> MILQIHSQNPHLLDLLNKNPHTDLGIYAKSLRNGQLIGNAVSAYQYDVVFQDTRYSYLPEESNQIDFQSYCSPLVILHICNEFFKELLQEKQTYWSQQIKWLERTRAEVDTYPCTIEVKNLYANSTWYSKGHFMMERYFKNIHITPIVGNNLSLRVEGKSVFEAMNLLSFIAVTTHITNTYGEYTYIDDHFAQKYARILTNIPQVPYFVFYLFIKRAIKSERQFAEIKPMFEAYFKEEGLDIDFQFTDTHGSRMDFIVKELGMEYPILDIGCGELKYYRRFMRRNYNYSHPYFATDTDKSVGDYAALLKERMEADNLYFFSDWTDYEYKNPVNIILTEVIEHNTPEAAEALVKHCLSLNFHKMIITTPNSLFNKYYFDEDPESLRHEDHHFEWTPQEFQDFIRHCVGDTSLEV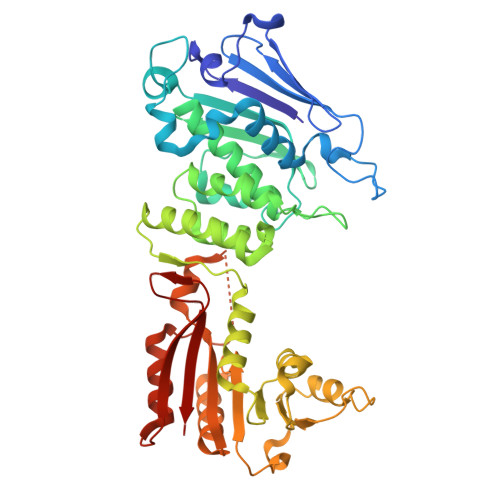TYCGIGDRINGETPTQAVVITRK7-[3-(aminomethyl)phenyl]-4-methylquinolin-2-amine | C17 H17 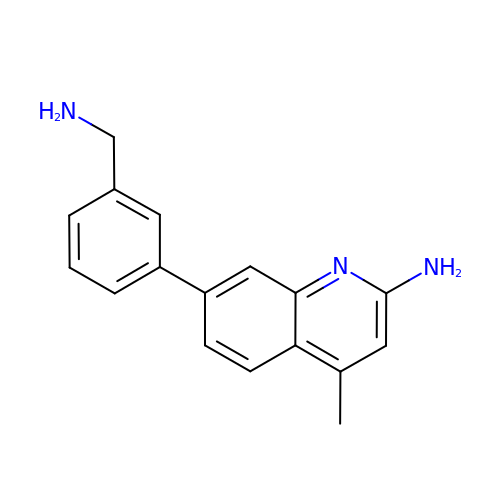N3 | IYZDGTYWMCMPLR-UHFFFAOYSA-N3-azanyloxy-2-[(~{E})-[2-methyl-3-oxidanyl-5-(phosphonooxymethyl)pyridin-4-yl]methylideneamino]propanoic acid 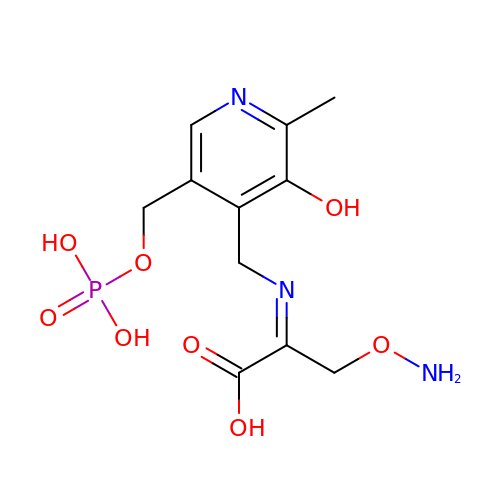| C11 H16 N3 O8 P | ICHYGZXBYNDCFX-NTEUORMPSA-N(5-chloro-3-methyl-1-benzothiophen-2-yl)acetic acid | C11 H9 Cl O2 S | 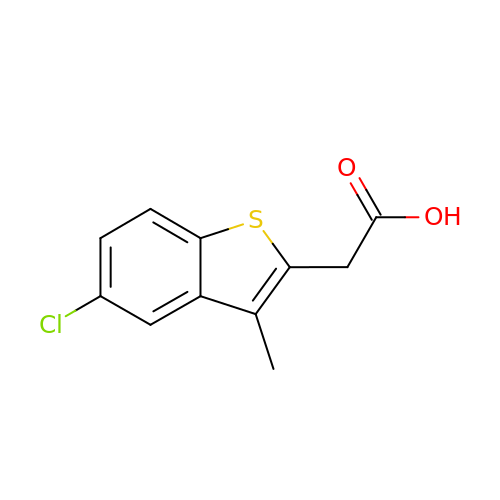QNJIHQOPIPJYLU-UHFFFAOYSA-N> ADKRAHHNALERKRRDHIKDSFHSLRDSVPSLQGEKASRAQILDKATEYIQYM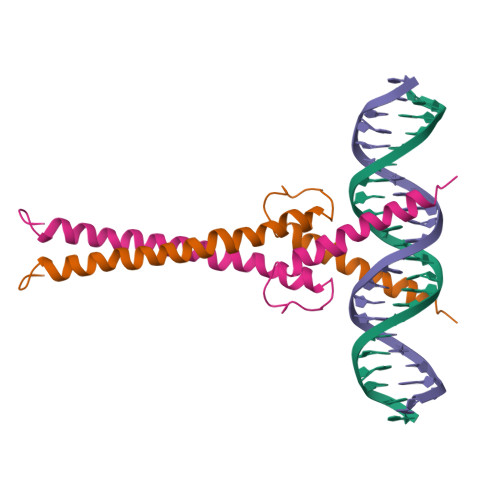RRKNHTHQQDIDDLKRQNALLEQQVRALEKARS> GHMHGRLKVKTSEEQAEAKRLEREQKLKLYQSATQAVFQKRQAGELDESVLELTSQILGANPDFATLWNCRREVLQHLETEKSPEESAALVKAELGFLESCLRVNPKSYGTWHHRCWLLSRLPEPNWARELELCARFLEADERNFHCWDYRRFVAAQAAVAPAEELAFTDSLITRNFSNYSSWHYRSCLLPQLHPQPDSGPQGRLPENVLLKELELVQNAFFTDPNDQSAWFYHRWLLGAGSGRCELSVEKSTVLQSELESCKELQELEPENKWCLLTIILLMRALDPLLYEKETLQYFSTLKAVDPMRAAYLDDLRSKFLLENSVLKMEYA;> GTQQKDVTIKSDAPDTLLLEKHADYIA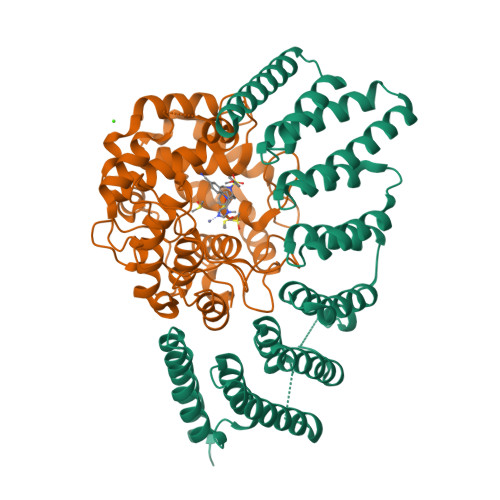SYGSKKDDYEYCMSEYLRMSGVYWGLTVMDLMGQLHRMNKEEILVFIKSCQHECGGVSASIGHDPHLLYTLSAVQILTLYDSIHVINVDKVVAYVQSLQKEDGSFAGDIWGEIDTRFSFCAVATLALLGKLDAINVEKAIEFVLSCMNFDGGFGCRPGSESHAGQIYCCTGFLAITSQLHQVNSDLLGWWLCERQLPSGGLNGRPEKLPDVCYSWWVLASLKIIGRLHWIDREKLRSFILACQDEETGGFADRPGDMVDPFHTLFGIAGLSLLGEEQIKPVSPVFCMPEEVLQRVNVQPELVS>SNATYQYNMNFEKLGKCIIINNKNFDKVTGMGVRNGTDKDAEALFKCFRSLGFDVIVYNDCSCAKMQDLLKKASEEDHTNAACFACILLSHGEENVIYGKDGVTPIKDLTAHFRGDRCKTLLEKPKLFFIQACRGTELDDGIQ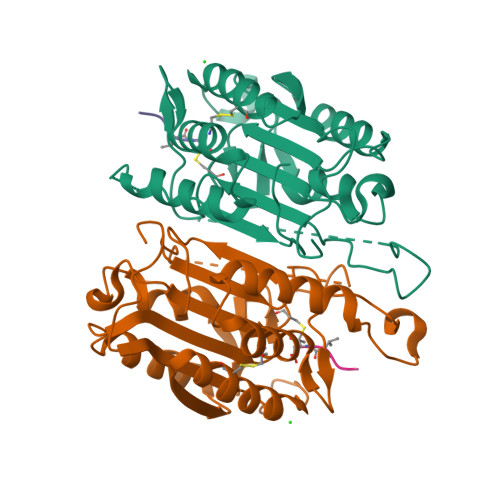AASGPINDTDANPRYKIPVEADFLFAYSTVPGYYSWRSPGRGSWFVQALCSILEEHGKDLEIMQILTRVNDRVARHFESQSDDPHFHEKKQIPCVVSMLTKELYFSQ[2x]The PriA enzyme is capable of operating in the L-histidine biosynthesis pathway as HisA, while also functioning in the L-tryptophan biosynthesis pathway as TrpF. The product of the priA gene, which is a hisA homolog, catalyzes two analogous isomerizations of structurally similar substrates: (i) the conversion of N-(5'-phosphoribosyl)-anthranilate (PRA) into 1-(O-carboxyphenylamino)-1'-deoxyribulose-5'-phosphate (CdRP) (TrpF or PRA isomerase activity); and (ii) the conversion of N-[(5-phosphoribosyl) formimino]-5-aminoimidazole-4-carboxamide ribonucleotide (ProFAR) into N-[(5-phosphoribulosyl)formimino]-5-aminoimidazole-4-carboxamide ribonucleotide (PRFAR) (HisA or ProFAR isomerase activity). Moreover, evolution of PriA in response to genome dynamics has lead to the appearance of the SubHisA and PriB subfamilies, which have been shown to have different substrate specificities. After the loss of constrictions imposed by the retention of biosynthetic pathways, we found that evolutionary patterns correlate with the sub-functionalization, yet not necessarily specialization, of PriA into two new subfamilies, which we named SubHisA2 and SubTrpF.

To potentially identify mutations in active-site residues that may affect kcat and KM parameters, we attempted to elucidate the structure of the five PriA homologs that we were able to in vitro characterize. However, we were only able to crystallize and solve the structure of PriA_Org15 (H1) at atomic resolution of 1.05 Å (PDB: 4 × 2R, Figure 7; Figure 7—source data 1). First, enzymes from Org15, Org21, and Org22 (H1) showed dual-substrate specificity but also poor catalytic efficiencies, namely, kcat/KMProFAR from 0.01 to 0.1 μM−1s−1 and kcat/KMPRA around 0.01 μM−1s−1. In the case of the H1 enzymes, the poor turnovers are compensated for by relatively high substrate affinities (KM), mainly for ProFAR. Since the loop contributing Trp139 and Arg137 is mostly disordered, and Arg137 itself does not adopt substrate binding-relevant position in the structure from A. urogenitalis, only the equivalent elements from the M. tuberculosis homolog are shown. In PriA, Gly126 faces the active site near the catalytic residue Asp128. Trp139 is important for the correct positioning of the catalytic residues present in loop 5, and for substrate binding through stacking interactions. Indeed, the indole group of Trp139 in PriAs can form a hydrogen bond with Asp128, stabilizing the knot-like conformation observed during ProFAR binding. Arg83 interacts with the second phosphate group of ProFAR, allowing its correct position in the substrate-binding pocket of PriA. An extra factor potentially hampering sequence and structural analysis is the higher-than-normal mutation rates of these protein sub-families, which translates into lack of sequence conservation and disordered regions in X-ray crystal structures.

> SNAMLTLLPAVDVADGKAVRLLQGEAGSETDYGSPIEAARDWVEAGAEWIHLVDLDAAFGRGSNAPLLERIVGEVGIKVELSGGIRDDASLTRALKAGAARVNLGTAALEDPQWTARVIAEHGEKIAVGLDVRGTTLAARGWTKEGGDLWQTLDRLNEAGCRRYVVTDVTKDGTLTGPNTELLRQVAARTSAPVVASGGISSLEDIAALARLVPQGVDSAIVGKALYNGNFTLPQALAVAGGAAVQDVQA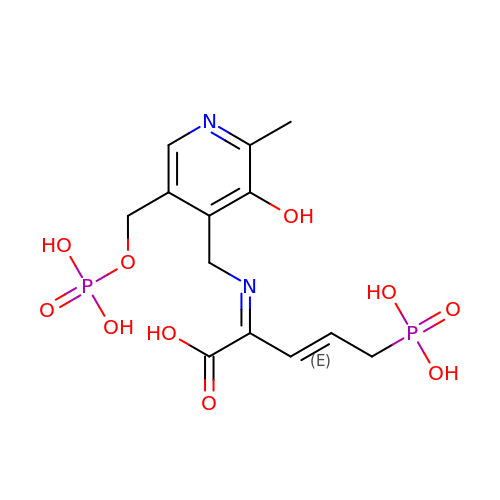2-[(3-HYDROXY-2-METHYL-5-PHOSPHONOOXYMETHYL-PYRIDIN-4-YLMETHYL)-IMINO]-5-PHOSPHONO-PENT-3-ENOIC ACID | C13 H18 N2 O10 P2 | VKWJKURKEYQKKW-ZCOJICPHSA-N3-(3-methylbutyl)-4~{H}-1,2,3-triazol-5-one 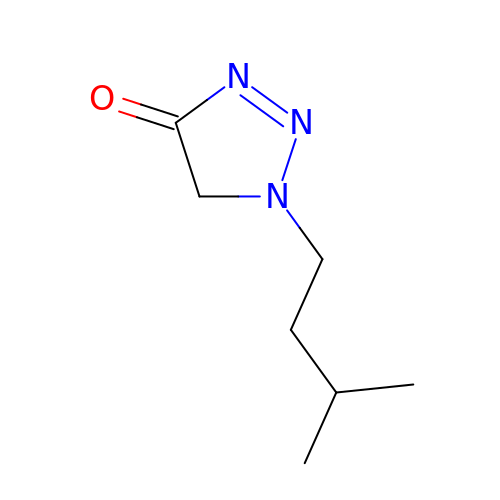| C7 H13 N3 O | NRFSJPLMHMLGTM-UHFFFAOYSA-N>MMVISEKVRKALNDQLNREIYSSYLYLSMATYFDAEGFKGFAHWMKKQAQEELTHAMKFYEYIYERGGRVELEAIEKPPSNWNGIKDAFEAALKHEEFVTQSIYNILELASLALDHATVSFLKWFVDEQV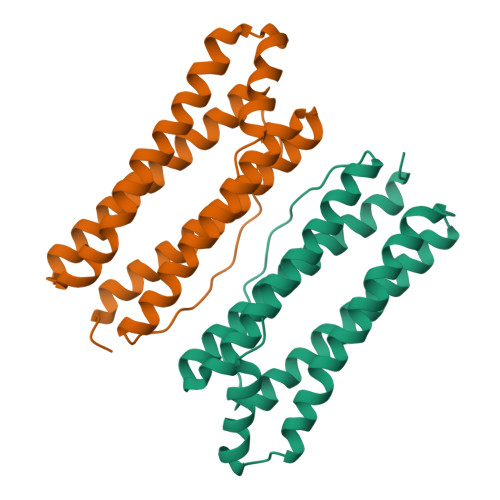EEEDQVREILDLLEKAFGQMSVIFQLDRYLGQRE[2x]> QSMEGNGPAAVHYQPASPPRDACVYSSCYSEENVWKLC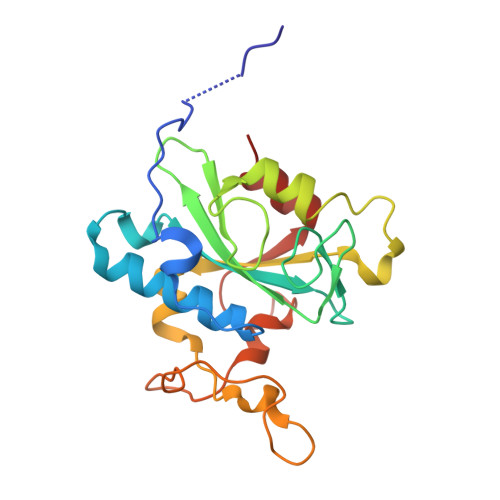EYIKNHDQYPLEECYAVFISNERKMIPIWKQQARPGDGPVIWDYHVVLLHVSSGGQSFIYDLDTVLPFPCLFDTYVEDAIKSDDDIHPQFRRKFRVICADSYLKNFASDRSHMKDSSGNWREPPPPYPCIETGDSKMNLNDFISMDPKVGWGAVYTLSEFTHRFGS>MDIKINDITLGNNSPFVLFGGINVLESLDSTLQTCAHYVEVTRKLGIPYIFKASFDKANR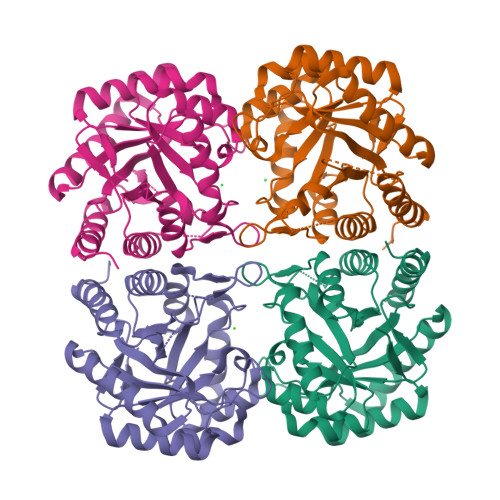SSIHSYRGVGLEEGLKIFEKVKAEFGIPVITDVHEPHQCQPVAEVCDVIQLPAFLAQQTDLVVAMAKTGNVVNIKKPQFLSPSQMKNIVEKFHEAGNGKLILCERGSSFGYDNLVVDMLGFGVMKQTCGNLPVIFDVTHSLQTRDAGSAASGGRRAQALDLALAGMATRLAGLFLESHPDPKLAKCDGPSALPLHLLEDFLIRIKALDDLIKSQPILTIE[4x]> FASPAPSNQGSSVFGAPA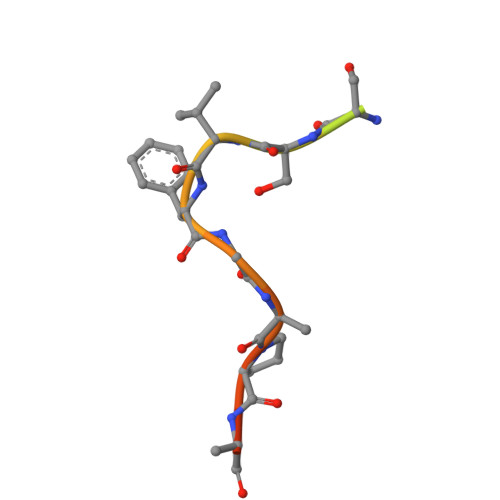QST>SMFIKKIKAKANNNEINVIIEIPMNSGPIKYEFDKESGALFVDRFMQTTMSYPCNYGFIPDTLSNDG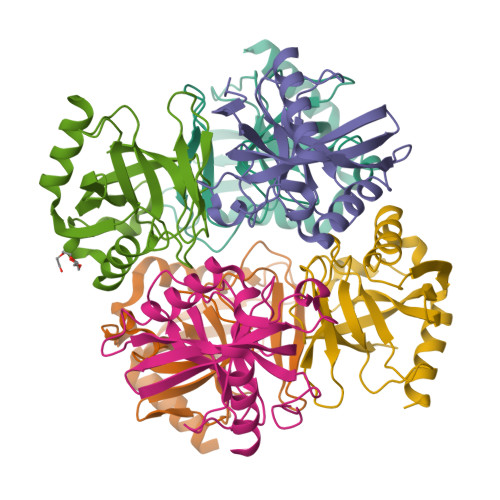DPVDVLVVAHHPVVPGSVIKCRAIGVLMMEDESGLDEKIIAVPTSKLDITFDHIKELDDLCEMLKKRIVHFFEHYKDLEKGKWVKVTGWGDKVKAETLIKEGIDRN[12x]>[6x]GSHMASMTGGQQMGRGSMRQFKVSHPGEMIARDLEDMGVSGRRFAHNIGV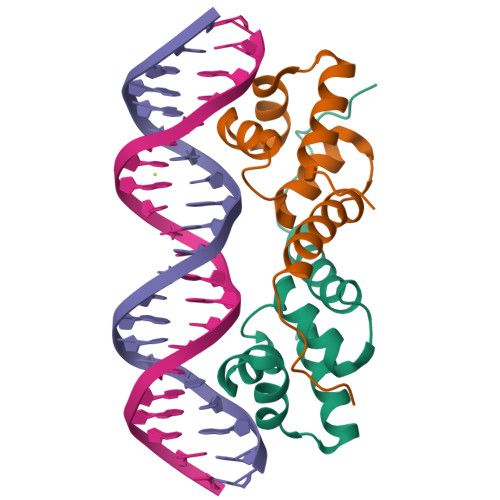TPATVSRLLAGKTALTPSLSIRIAAALGSTPEFWLRLQSNYDLRQLENQIDTSGIVLYGESNEQQQNAQEH> MKSNDMNITVELTFFEPYRLVEWFDWDARKKSHSAMRGQAFAQWTWKGKGRTAGKSFITGTLVRSAVIKAVEELLSLNNGKWEGVPCCNGSFQTDESKGKKPSFLRKRHTLQWQANNKNICDKEEACPFCILLGRFDNAGKVHERNKDYDIHFSNFDLDHKQEKNDLRLVDIASGRILNRVDFDTGKAKDYFRTWEADYETYGTYTGRITLRNEHAKKLLLASLGFVDKLCGALCRIEVIKKSESPLPSDTKEQSYTKDDTVEVLSEDHNDELRKQAEVIVEAFKQNDKLEKIRILADAIRTLRLHGEGVIEKDELPDGKEERDKGHHLWDIKVQGTALRTKLKELWQSNKDIGWRKFTEMLGSNLYLIYKKETGGVSTRFRILGDTEYYSKAHDSEGSDLFIPVTPPEGIETKEWIIVGRLKAATPFYFGVQQPSDSIPGKEKKSEDSLVINEHTSFNILLDKENRYRIPRSALRGALRRDLRTAFGSGCNVSLGGQILCNCKVCIEMRRITLKDSVSDFSEPPEIRYRIAKNPGTATVEDGSLFDIEVGPEGLTFPFVLRYRGHKFPEQLSSVIRYWEENDGKNGMAWLGGLDSTGKGRFAL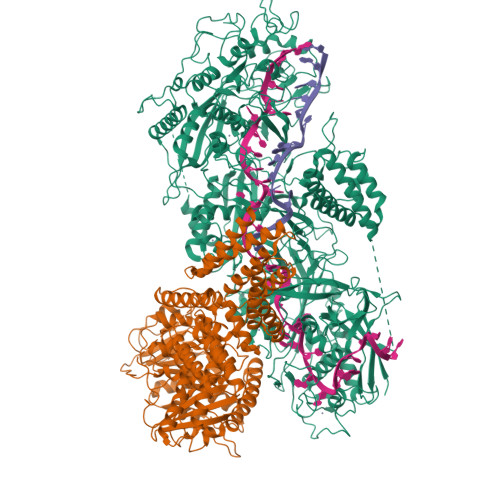KDIKIFEWDLNQKINEYIKERGMRGKEKELLEMGESSLPDGLIPYKFFEERECLFPYKENLKPQWSEVQYTIEVGSPLLTADTISALTEPGNRDAIAYKKRVYNDGNNAIEPEPRFAVKSETHRGIFRTAVGRRTGDLGKEDHEDCTCDMCIIFGNEHESSKIRFEDLELINGNEFEKLEKHIDHVAIDRFTGGALDKAKFDTYPLAGSPKKPLKLKGRFWIKKGFSGDHKLLITTALSDIRDGLYPLGSKGGVGYGWVAGISIDDNVPDDFKEMINKTEMPLPEEVEESNNGPINNDYVHPGHQSPKQDHKNKNIYYPHYFLDSGSKVYREKDIITHEEFTEELLSGKINCKLETLTPLIIPDTSDENGLKLQGNKPGHKNYKFFNINGELMIPGSELRGMLRTHFEALTKSCFAIFGEDSTLSWRMNADEKDYKIDSNSIRKMESQRNPKYRIPDELQKELRNSGNGLFNRLYTSERRFWSDVSNKFENSIDYKREILRCAGRPKNYKGGIIRQRKDSLMAEELKVHRLPLYDNFDIPDSAYKANDHCRKSATCSTSRGCRERFTCGIKVRDKNRVFLNAANNNRQYLNNIKKSNHDLYLQYLKGEKKIRFNSKVITGSERSPIDVIAELNERGRQTGFIKLSGLNNSNKSQGNTGTTFNSGWDRFELNILLDDLETRPSKSDYPRPRLLFTKDQYEYNITKRCERVFEIDKGNKTGYPVDDQIKKNYEDILDSYDGIKDQEVAERFDTFTRGSKLKVGDLVYFHIDGDNKIDSLIPVRISRKCASKTLGGKLDKALHPCTGLSDGLCPGCHLFGTTDYKGRVKFGFAKYENGPEWLITRGNNPERSLTLGVLESPRPAFSIPDDESEIPGRKFYLHHNGWRIIRQKQLEIRETVQPERNVTTEVMDKGNVFSFDVRFENLREWELGLLLQSLDPGKNIAHKLGKGKPYGFGSVKIKIDSLHTFKINSNNDKIKRVPQSDIREYINKGYQKLIEWSGNNSIQKGNVLPQWHVIPHIDKLYKLLWVPFLNDSKLEPDVRYPVLNEESKGYIEGSDYTYKKLGDKDNLPYKTRVKGLTTPWSPWNPFQVIAEHEEQEVNVTGSRPSVTDKIERDGKMV;> MNNTEENIDRIQEPTREDIDRKEAERLLDEAFNPRTKPVDRKKIINSALKILIGLYKEKKDDLTSASFISIARAYYLVSITILPKGTTIPEKKKEALRKGIEFIDRAINKFNGSILDSQRAFRIKSVLSIEFNRIDREKCDNIKLKNLLNEAVDKGCTDFDTYEWDIQIAIRLCELGVDMEGHFDNLIKSNKANDLQKAKAYYFIKKDDHKAKEHMDKCTASLKYTPCSHRLWDETVGFIERLKGDSSTLWRDFAIKTYRSCRVQEKETGTLRLRWYWSRHRVLYDMAFLAVKEQADDEEPDVNVKQAKIKKLAEISDSLKSRFSLRLSDMEKMPKSDDESNHEFKKFLDKCVTAYQDGYVINRSEDKEGQGENKSTTSKQPEPRPQAKLLELTQVPEGWVVVHFYLNKLEGMGNAIVFDKCANSWQYKEFQYKELFEVFLTWQANYNLYKENAAEHLVTLCKKIGETMPFLFCDNFIPNGKDVLFVPHDFLHRLPLHGSIENKTNGKLFLENHSCCYLPAWSFASEKEASTSDEYVLLKNFDQGHFETLQNNQIWGTQSVKDGASSDDLENIRNNPRLLTILCHGEANMSNPFRSMLKLANGGITYLEILNSVKGLKGSQVILGACETDLVPPLSDVMDEHYSVATALLLIGAAGVVGTMWKVRSNKTKSLIEWKLENIEYKLNEWQKETGGAAYKDHPPTFYRSIAFRSIGFPL>RRNMFQGIEDPDRIERAFNLPLYGLVPQSAEQVKLDAQAEKSGSRTRPILASLRPKDLSVESLRSLRTAMQFAMMDAKNRVIVLTGPTPGIGKSFLTVNLAVLLAHSGKRVLLIDADMRRGLLDRYFGLTSQPGLSELLSDQSALEDAVRETPVQGLSFISAGTRPPNPSELLMSTRLPQYLEGLGKRYDVVLIDSPPVLAVTDATIIGRMAGSTFLVLRSGMHTEGEIADAIKRLRTAGVDLEGGIFNGVPPKARGYGRGYAAVHEYLSA[2x]

BceF is a bacterial tyrosine kinase (BY-kinase) from Burkholderia cepacia, a Gram-negative bacterium accountable for respiratory infections in immunocompromised and cystic fibrosis patients. BceF is involved in the production of exopolysaccharides secreted to the biofilm matrix and promotes resistant and aggressive infections. Similar to other BY-kinases in Gram-negative bacteria, BceF is composed of a short cytoplasmic N-terminus, followed by a transmembrane helix, a periplasmic/extracellular domain, a second transmembrane helix, and a cytoplasmic C-terminal catalytic domain. The catalytic cytoplasmic domain contains the Walker A, Walker A’ and Walker B motifs that are also found in ATPases of the MinD/Mrp superfamily.

The crystal structure of B. cepacia BceF kinase domain, overexpressed and purified from E. coli, was determined at 1.85Å resolution. The plasmid construct used encompassed the BceF kinase domain, i.e., residues 471–741. The structure features a fold similar to other BY-kinases of known structures, showing a central, eight-stranded curved β-sheet, flanked by 12 helices of varying lengths. In the crystallographic asymmetric unit, there are two virtually identical kinase domains of BceF, with a root-mean-square deviation (RMSD) of 0.36 Å across 241 paired residues. The structure revealed an adenosine diphosphate (ADP) molecule bound at the active site, probably co-purified from the bacteria, since it was not added during the purification or crystallization of BceF. The catalytic pocket exhibits the ATP-binding motifs common to BY-kinases and other nucleotide-binding proteins, including Walker A (residues 556GPTPGIGKS564), Walker A’ (residues 585DAD587), and Walker B (residues 661VVLID665). The active site pocket in BceF, with side chains closer than 4 Å to the ADP molecule, includes the highly conserved Pro497, Ser499, Gln502, Ile561, Lys563, Ser564, Phe565, Arg590, and Asn719 residues, along with the moderate evolutionary conserved Gln498, Pro559, Arg690, and the evolutionary variable Asp506 and Arg517 residues. Of note, Arg590 is facing the active site only in one of the BceF molecules in the asymmetric unit (chain A), but not in the other. In contrast, the interface of the dimer observed in the crystal packing of the BceF kinase domain was not evolutionary conserved. If the BceF kinase domain dimer observed in solution has the same arrangement observed in the crystal form, the partial obstruction of the active sites by the interface might explain the low enzymatic efficiency observed.> GLIVDTRDVEERVHVMRKTKLAPTVAHGVFNPEFGPAALSNKDPRLNEGVVLDEVIFSKHKGDTKMSAEDKALFRRCAADYASRLHS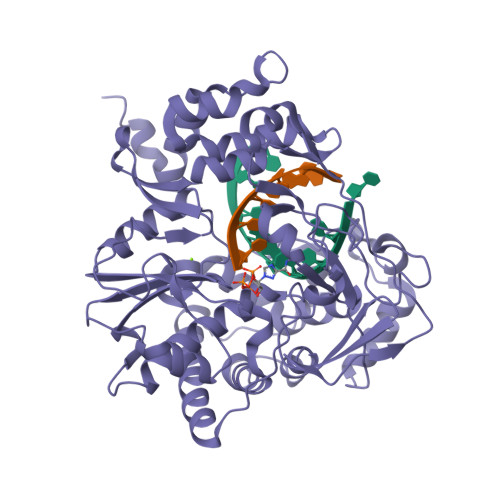VLGTANAPLSIYEAIKGVDGLDAMEPDTAPGLPWALQGKRRGALIDFENGTVGPEVEAALKLMEKREYKFACQTFLKDEIRPMEKVRAGKTRIVDVLPVEHILYTRMMIGRFCAQMHSNNGPQIGSAVGCNPDVDWQRFGTHFAQYRNVWDVDYSAFDANHCSDAMNIMFEEVFRTEFGFHPNAEWILKTLVNTEHAYENKRITVEGGMPSGCSATSIINTILNNIYVLYALRRHYEGVELDTYTMISYGDDIVVASDYDLDFEALKPHFKSLGQTITPADKSDKGFVLGHSITDVTFLKRHFHMDYGTGFYKPVMASKTLEAILSFARRGTIQEKLISVAGLAVHSGPDEYRRLFEPFQGLFEIPSYRSLYLRWVNAVCGDAAALEHH>[3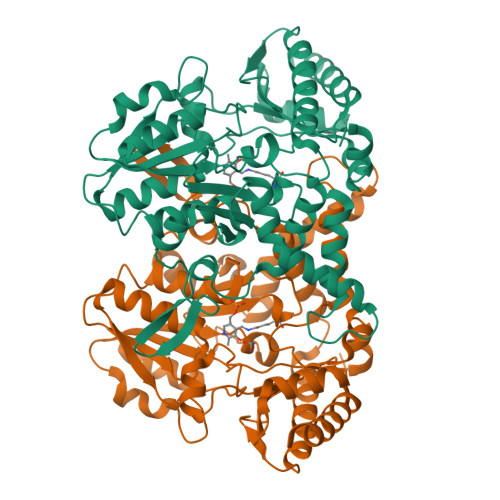x]GSHMNVFNPAQFRAQFPALQDAGVYLDSAATALKPEAVVEATQQFYSLSAGNVHRSQFAEAQRLTARYEAAREKVAQLLNAPDDKTIVWTRGTTESINMVAQCYARPRLQPGDEIIVSVAEHHANLVPWLMVAQQTGAKVVKLPLNAQRLPDVDLLPELITPRSRILALGQMSNVTGGCPDLARAITFAHSAGMVVMVDGAQGAVHFPADVQQLDIDFYAFSGHKLYGPTGIGVLYGKSELLEAMSPWLGGGKMVHEVSFDGFTTQSAPWKLEAGTPNVAGVIGLSAALEWLADYDINQAESWSRSLATLAEDALAKRPGFRSFRCQDSSLLAFDFAGVHHSDMVTLLAEYGIALRAGQHCAQPLLAELGVTGTLRASFAPYNTKSDVDALVNAVDRALELLVD>MSLKTTTSSTPSDRITWVRISSCYLPLATPISDAKVLTGRQKPMTEIAILFAEIETAGGHQGLGFSYSKRAGGPGQFAHAREIAPALIGEDPSDIAKLWDKLCWAGASAGRSGLSTQAIGAFDVALWDLKAKRAGLSLAKLLGSYRDSVRCYNTSGGFLHTPIDQLMVNASASIERGIGGIKLKVGQPDGALDIARVTAVRKHLGDAVPLMVDANQQWDRPTAQRMCRIFEPFNLVWIEEPLDAYDHEGHAALALQFDTPIATGEMLTSAAEHGDLIRHRAADYLMPDAPRVGGITPFLKIASLAEHAGLMLAPHFAMELHVHLAAAYPREPWVEHFEWLEPLFNERIEIRDGRMLVPTRPGLGL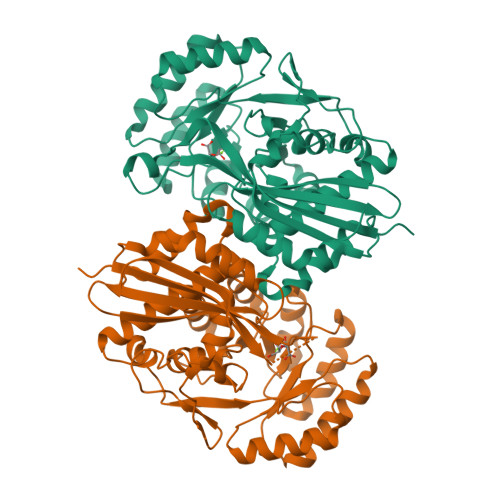TLSGQVKAWTREEAQVGTRPEGHHHHHH[4x]In budding yeast, the TREX2 complex binds to NPCs and is thought to function in integrating the nuclear export of mature transcripts with earlier steps in the gene expression pathway, together with promoting genome stability through inhibiting R-loop formation (1–4). TREX2 is constructed from a Sac3 scaffold to which Thp1, Sem1, Cdc31 and two Sus1 chains bind. Sus1 and Cdc31 bind to the Sac3 centrin binding (CID) region (Sac3CID, residues 723–805) that has an unusually long α-helix about which the other three chains coil. We report here the crystal structure of the interface between TREX2 and Nup1 that shows that Nup1 residues 330–340 bind primarily to a cavity formed between the Sac3 helix (residues 757–777) and the Sus1 chain closest to Cdc31 (Sus1B) and show that Phe336Nup1 and Phe338Nup1 are crucial for this interaction.

Crystals with P3221 symmetry that diffracted to 3.0 Å resolution were obtained from a solution containing Nup1322–355 and Sac3757–787:Sus1B and crystals with P21 symmetry that diffracted to 2.6Å resolution were obtained with Nup1316–340 and the Sac3753–805:Sus1B:Cdc31 complex. Molecular replacement using appropriate search models derived from the Sac3CID domain complex showed clear difference density due to the Nup1 fragment, with the side chains of Phe336 and Phe338 being especially clear. For the P21 crystals, Nup1 residues 330–339 were easily built, but density for residues 316–329 was not observed, even after repeated cycles of refinement and rebuilding. After refinement, additional weak density was observed between the N- and C-terminal helices of each Sus1 chain that appeared to be due to a second weakly bound peptide chain that was tentatively assigned to Nup1 residues 326–330. Vague density was visible in the place assigned to Nup1 residues 326–331 in the P21 crystal and it appears that in both crystals an additional Nup1 peptide chain became bound at this site. In both cases, the density due to this additional peptide chain was poor, consistent with it being bound weakly and/or sub-stoichiometrically and is likely the result of the peptide being present in molar excess during crystallogenesis, indicating that the binding of this second Nup1 chain was likely a crystallisation artefact. In the final model of both complexes, the structural arrangement of Sus1B bound to Sac3 and Cdc31 bound to Sac3 was essentially unaltered from that observed in the absence of Nup1 (17), consistent with Nup1 binding not generating a substantial conformational change. In both crystals, the principal Nup1 binding site was based on a cavity formed by Sus1B helices α1 and α2 and residues 757–787 of the Sac3CID domain helix. The Nup1 chain adopted an unstructured conformation and the interaction was dominated by burying the aromatic side chains of Phe336Nup1 and Phe338Nup1. The interior of the binding cavity contained two deeper hydrophobic clefts into which the aromatic side chains of Phe336Nup1 and Phe338Nup1 fitted snugly.

>[2x]MSKNRSSLQSGPLNSELLEEQKQEIYEAFSLFDMNNDGFLDYHELKVAMKALGFELPKREILDLIDEYDSEGRHLMKYDDFYIVMGEKILKRDPLDEIKRAFQLFDDDHTGKISIKNLRRVAKELGETLTDEELRAMIEEFDLDGDGEINENEFIAICTDS;>EANYRKDFIDTMTRELYDAFLHERLYLIYMDSRAELKRNSTLKKKFFEKWQAS[2x];>MTMDTAQLKSQIQQYLVESGNYELISNELKARLLQEGWVDKVKDLTKSEMNINESTNFTQILSTVEPKALEMVSDSTRETVLKQIREFLEEIVDTQ[2x];>LKKNIEPKKDKESIVLPTVGFDFIK[4x]> MTPILAAEALTYAFPGGVKALDDLSLAVPKGESLAILGPNGAGKSTLLLHLNGTLRPQSGRVLLGGTATGHSRKDLTGWRRRVGLVLQDADDQLFATTVFEDVSFGPLNLGLSEAEARARVEEALAALSISDLRDRPTHMLSGGQKRRVAIAGAVAMRPEVLLLDEPTAGLDLAGTEQLLTLLRGLRAAGMTLVFSTHDVELAAALADRVALFRTGRVLAEGAAEAVLSDRATLAKVALRPP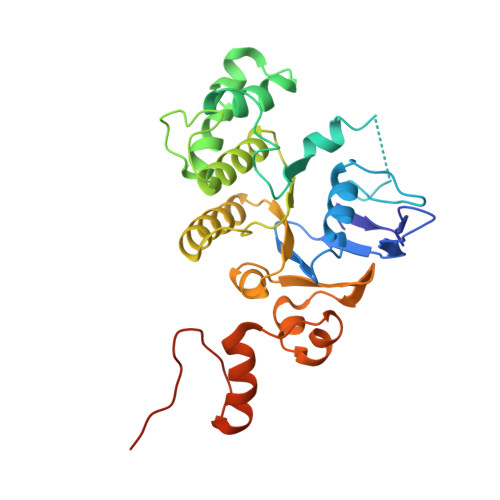LVIDLALLARDHGLLAPEAPLPKTRDALAAQMAGWTRR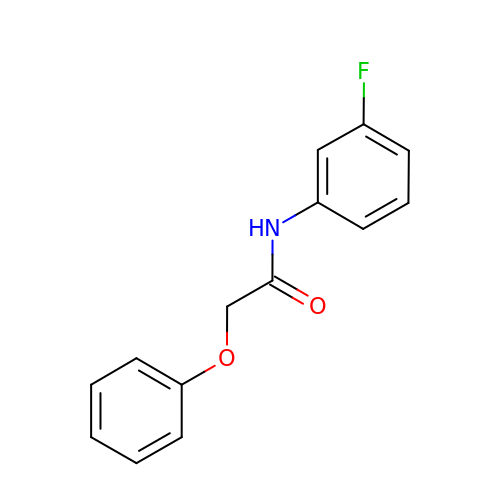N-(3-fluorophenyl)-2-phenoxyacetamide | C14 H12 F N O2 | VTCNQCNGFQNSAO-UHFFFAOYSA-N>[2x]DDHSELLVNTKSGKVMGTRVPVLSSHISAFLGIPFAEPPVGNMRFRRPEPKKPWSGVWNASTYPNNCQQYVDEQFPGFSGSEMWNPNREMSEDCLYLNIWVPSPRPKSTTVMVWIYGGGFYSGSSTLDVYNGKYLAYTEEVVLVSLSYRVGAFGFLALHGSQEAPGNVGLLDQRMALQWVHDNIQFFGGDPKTVTIFGESAGGASVGMHILSPGSRDLFRRAILQSGSPNCPWASVSVAEGRRRAVELGRNLNCNLNSDEELIHCLREKKPQELIDVEWNVLPFDSIFRFSFVPVIDGEFF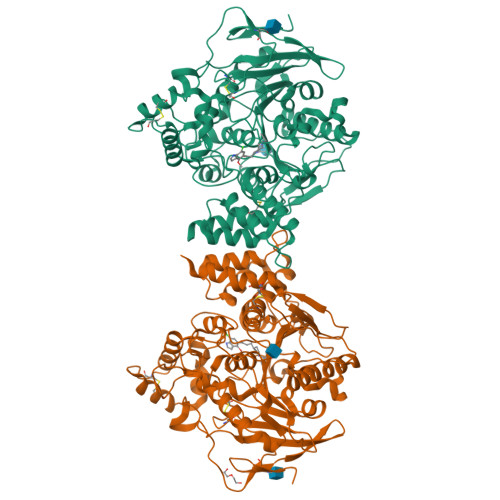PTSLESMLNSGNFKKTQILLGVNKDEGSFFLLYGAPGFSKDSESKISREDFMSGVKLSVPHANDLGLDAVTLQYTDWMDDNNGIKNRDGLDDIVGDHNVICPLMHFVNKYTKFGNGTYLYFFNHRASNLVWPEWMGVIHGYEIEFVFGLPLVKELNYTAEEEALSRRIMHYWATFAKTGNPNEPHSQESKWPLFTTKEQKFIDLNTEPMKVHQRLRVQMCVFWNQFLPKLLNATAC>MNGVLIPHTPIAVDFWSLRRAGTARLFFLSHMHSDHTVGLSSTWARPLYCSPITAHLLHRHLQVSKQWIQALEVGESHVLPLDEIGQETMTVTLLDANHCPGSVMFLFEGYFGTILYTGDFRYTPSMLKEPALTLGKQIHTLYLDNTNCNPALVLPSRQEAAHQIVQLIRKHPQHNIKIGLYSLGKESLLEQLALEFQTWVVLSPRRLELVQLLGLADVFTVEEKAGRIHAVDHMEICHSNMLRWNQTHPTIAILPTSRKIHSSHPDIHVIPYSDHSSYSELRAFVAALKPCQVVPIVSRRPCG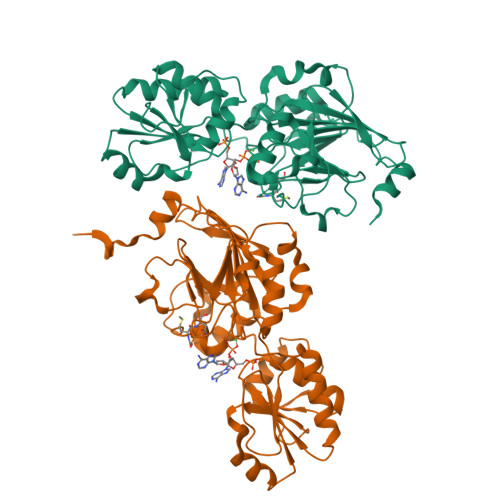GFQDSLSPRISVPLIPDSVQQYMSSSSRKPSAENLYFQ[2x]>[6x]DADKLPHTKVTLVAPPQVHPHEQATKSGPKVVEFTMTIEEKKMVIDDKGTTLQAMTFNGSMPGPTLVVHEGDYVQLTLVNPATNAMPHNVDFHGATGALGGAKLTNVNPGEQATLRFKADRSGTFVY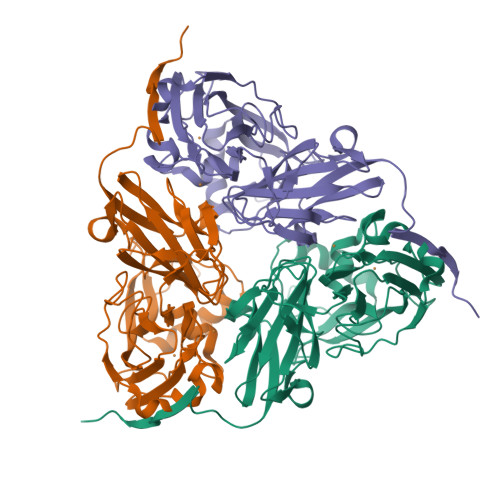HCAPEGMVPWHVVSGLSGTLMVLPRDGLKDPQGKPLHYDRAYTIGEFDLYIPKGPDGKYKDYATLAESYGDTVQVMRTLTPSHIVFNGKVGALTGANALTAKVGETVLLIHSQANRDTRPHLIGGHGDWVWETGKFANPPQRDLETWFIRGGSAGAALYTFKQPGVYAYLNHNLIEAFELGAAGHIKVEGKWNDDLMKQIKAPAPIPR> GPAEEEMSNELQNLDVQGKSKATGTGLVYVDAFTRFHCLWDASHPEC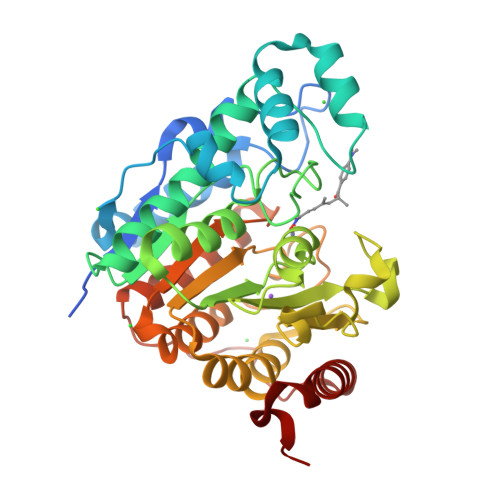PARVSTVMEMLETEGLLGRCVQVEARAVTEDELLLVHTKEYVELMKSTQNMTEEELKTLAEKYDSVYLHPGFFSSACLSVGSVLQLVDKVMTSQLRNGFSINRPPGHHAQADKMNGFCMFNNLAIAARYAQKRHRVQRVLIVDWDVHHGQGIQYIFEEDPSVLYFSVHRYEDGSFWPHLKESDSSSVGSGAGQGYNINLPWNKVGMESGDYITAFQQLLLPVAYEFQPQLVLVAAGFDAVIGDPKGGMQVSPECFSILTHMLKGVAQGRLVLALEGGYNLQSTAEGVCASMRSLLGDPCPHLPSSGAPCESALKSISKTISDLYPFWKSLQTF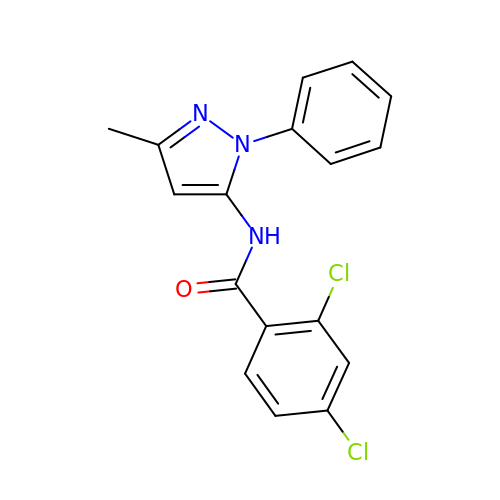2,4-dichloro-N-(3-methyl-1-phenyl-1H-pyrazol-5-yl)benzamide | C17 H13 Cl2 N3 O | AJPLAFYBSJYISV-UHFFFAOYSA-N>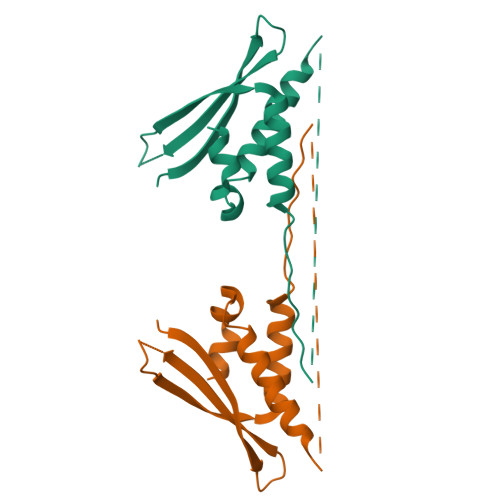 GSMSRQAKDDFLRHYTVSDPRTHPKGYTEYKVTAQFISKKDPEDVKEVVVWKRYSDFRKLHGDLAYTHRNLFRRLEEFPAFPRAQVFGRFEASVIEERRKGAEDLLRFTVHIPALNNSPQLKEFFRGG Speckle-type POZ protein (SPOP) is a ubiquitin ligase adaptor that binds substrate proteins and facilitates their proteasomal degradation. SPOP is composed of three domains: the meprin and tumor necrosis factor receptor-associated factor homology (MATH) substrate-interaction domain and two dimerization domains, bric à brac, tramtrack, broad complex and bric à brac, tramtrack, broad complex and C-terminal Kelch. Among the regulatory signals that control Pdx1 stability and function is a degradation pathway wherein Pdx1 associates with a ubiquitin ligase adaptor, speckle-type POZ protein (SPOP). Notably, neither SB motif in Pdx1 conforms to the established SB consensus sequence, but high-resolution structural characterization suggests that the Pdx1 SB motifs share a binding mode with other substrates.

We also present, to our knowledge, the first X-ray structure of SPOP-MATH without bound substrate. F102, W131, and F133 are frequently mutated in prostate cancers, which results in reduced affinity of SPOP for substrate proteins. There is no evidence to suggest that global structural changes contribute substantially to the energetics of binding, as comparison between substrate-bound and substrate-unbound SPOP–MATH structures reveals only minor side chain conformational changes upon substrate binding. In the structure of unbound SPOP–MATH, the electron density maps support modeling of Y123 in two different positions, but in substrate-bound structures, the residue instead adopts a single conformation.

> GPGKVVKFSYMWTINNFSFCREEMGEVIKSSTFSSGANDKLKWCLRVNPKGLDEESKDYLSLYLLLVSCPKSEVRAKFKFSILNAKGEETKAMESQRAYRFVQGKDWGFKKFIRRDFLLDEANGLLPDDKLTLFCEVSVVQD> MALPAHSLVMSSPALPAFLLCSTLLVIKMYVVAIITGQVRLRKKAFANPEDALRHGGPQYCRSDPDVERCLRAHRNDMETIYPFLFLGFVYSFLGPNPFVAWMHFLVFLVGRVAHTVAYLGKLRAPIRS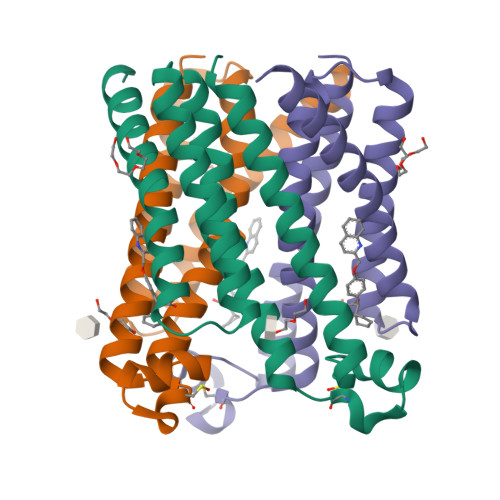VTYTLAQLPCASMALQILWEAARHL>MIVILDNGGQYVHRIHRSLKYIGVSSKIVPNTTPLEEIESNKEVKGIILSGGPDIEKAKNCIDIALNAKLPILGICLGHQLIALAYGGEVGRAEAEEYALTKVY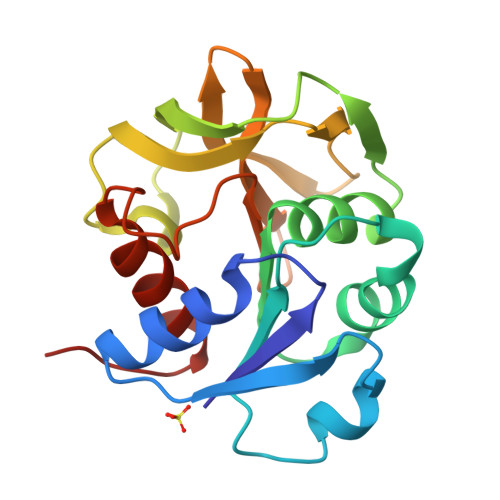VDKENVLFKNVPREFNAWASHKDEVKKVPEGFEILAHSDICQVEAMLHKTKPIYGVQFHPEVAHTEYGNEILKNFCKVCGYKFE[4x]>GPGRAKIDVDSVDHTDDYIHLRKWIKRIGIILRISGHWPFRLPHEKRNQHKSKFRQVYSCLVITLGFITCSCYCIGLCLSESIAQALNNITVTSYFLQSCVCYVSFIINSRKLETLFNYLFENEVVGCPRGYKMSSIKTTLFRCKFVAFSLGILSFFGWLMWTLLPLAVLVVDSGATGGGNQTSLRFVEAWYPFDTTTSPMNEVIAIYEAVAMIFLITAPMSSDIMFCVLMIFIVEHLKCLGMAIECTLKGISTNQHQNIGFDDSVSDVNVQRRIVIGKESPIQSIHVPIKECSRQSSDAVFREKRHGTHHQIIRSHNYTDATSLCNIVDSHVKIYRTMEIVQSVYSSYFATLFFTSCLAVCALAYFLAATSTSFTRVPGMVLYLMYIFLRIFLLCLLATEVAEQGLNLCHAGYSSKLVLASDHVRSTIQAIATRAQIPLSITGARFFTVNLSFLASMAGVMLTYFIVLLQVNAKPKP[4x]

MhORs thus autonomously assemble as homotetrameric odorant-gated ion channels and display the divergent chemical tuning profiles typical of this receptor family. Using cryo-electron microscopy, we elucidated the structure of MhOR5 in multiple gating states, alone and in complex with two of its agonists—the odorant eugenol and the insect repellent DEET. As in Orco, each MhOR5 subunit contributes a single helix (S7b) to the central ion conduction pathway, and their S0–S6 helices form a loosely packed domain that projects radially away from the pore axis.

To investigate the diversity of binding modes used by different ligands, we determined the 2.9 Å structure of MhOR5 in complex with the insect repellent DEET. The S7b helices in the DEET-bound structure were dilated to a diameter of 8.7 Å, indicating that different ligands elicit a common conformational change to gate the pore. Density corresponding to DEET localized to the same binding pocket as eugenol, encased within the same box-like configuration of aromatic and aliphatic side chains. As with eugenol, computational docking of DEET yielded multiple poses with comparable docking scores that fit the experimental density well. Whereas each of the top poses was predicted to adopt a distinct orientation, all were stabilized through a similar complement of hydrophobic and/or π-stacking interactions. The constellation of amino acids lining the binding pocket retains the same overall geometry in both structures, leaving the architecture of the hydrophobic box largely unchanged. However, a small displacement of the S4 helix results in expansion of the pocket, probably to accommodate the longer aliphatic moiety of DEET and avoid a steric clash with the side chain of Met209. Mutation of Met209 to smaller hydrophobic amino acids (valine or alanine) enhanced the affinity of DEET. Conversely, mutation of Ile213, another aliphatic S4 residue that lies in close proximity to DEET, to the larger residue methionine abolished DEET sensitivity but marginally altered eugenol signalling. Binding of DEET to the same site offers structural corroboration that this insect repellent might exploit the promiscuity of diverse ORs and serve as a molecular ‘confusant’ by scrambling the olfactory code.> MGSSHHHHHHSQDPNSSMVKWYYKTITFLPELCNNESLAAKCLRVLHGFNYQYET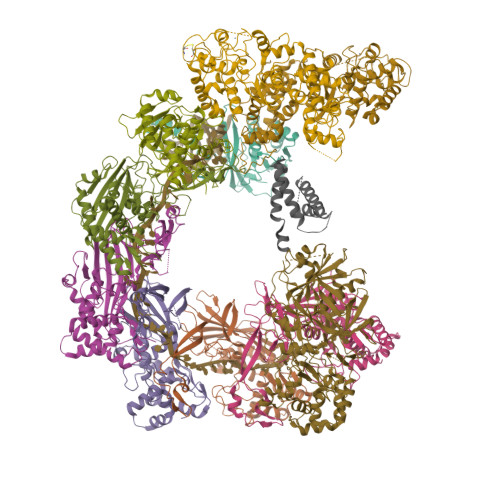RNIGVSFPLWCDATVGKKISFVSKNKIELDLLLKQHYFVQMEQLQYFHISNTVLVPEDCTYVSFRRCQSIDKLTAAGLARKIRRLEKRALSRGEQFDPSSFAQKEHTAIAHYHSLGESSKQTNRNFRLNIRMLSEQPREGNSIFSSYGLSNSENSFQPVPLI;> MQTLKELIASNPDDLTTELKRAFRPLTPHIAIDGNELDALTILVNLTDKTDDQKDLLDRAKCKQKLRDEKWWASCINCVNYRQSHNPKFPDIRSEGVIRTQALGELPSFLLSSSKIPPYHWSYSHDSKYVNKSAFLTNEFCWDGEISCLGELLKDADHPLWNTLKKLGCSQKTCKAMAKQLADITLTTINVTLAPNYLTQISLPDSDTSYISLSPVASLSMQSHFHQRLQDENRHSAITRFSRTTNMGVTAMTCGGAFRMLKSGAKFSSPPHHRLNSKRSWLTSEHVQSLKQYQRLNKSLIPENSRIALRRKYKIELQNMVRSWFAMQDHTLDSNILIQHLNHDLSYLGATKRFAYDPAMTKLFTELLKRELSNSINNGEQHTNGSFLVLPNIRVCGATALSSPVTVGIPSLTAFFGFVHAFERNINRTTSSFRVESFAICVHQLHVEKRGLTAEFVEKGDGTISAPATRDDWQCDVVFSLILNTNFAQHIDQDTLVTSLPKRLARGSAKIAIDDFKHINSFSTLETAIESLPIEAGRWLSLYAQSNNNLSDLLAAMTEDHQLMASCVGYHLLEEPKDKPNSLRGYKHAIAECIIGLINSITFSSETDPNTIFWSLKNYQNYLVVQPRSINDETTDKSSL;>[6x]MADLKLPTNLAYERSIDPSDVCFFVVWPDDRKTPLTYNSRTLLGQMEAASLAYDVSGQPIKSATAEALAQGNPHQVDFCHVPYGASHIECSFSVSFSSELRQPYKCNSSKVKQTLVQLVELYETKIGWTELATRYLMNICNGKWLWKNTRKAYCWNIVLTPWPWNGEKVGFEDIRTNYTSRQDFKNNKNWSAIVEMIKTAFSSTDGLAIFEVRATLHLPTNAMVRPSQVFTEKESGSKSKSKTQNSRVFQSTTIDGERSPILGAFKTGAAIATIDDWYPEATEPLRVGRFGVHREDVTCYRHPSTGKDFFSILQQAEHYIEVLSANKTPAQETINDMHFLMANLIKGGMFQHKGD;>[2x]MFLQRPKPYSDESLESFFIRVANKNGYGDVHRFLEATKRFLQDIDHNGYQTFPTDITRINPYSAKNSSSARTASFLKLAQLTFNEPPELLGLAINRTNMKYSPSTSAVVRGAEVFPRSLLRTHSIPCCPLCLRENGYASYLWHFQGYEYCHSHNVPLITTCSCGKEFDYRVSGLKGICCKCKEPITLTSRENGHEAACTVSNWLAGHESKPLPNLPKSYRWGLVHWWMGIKDSEFDHFSFVQFFSNWPRSFHSIIEDEVEFNLEHAVVSTSELRLKDLLGRLFFGSIRLPERNLQHNIILGELLCYLENRLWQDKGLIANLKMNALEATVMLNCSLDQIASMVEQRILKPNRKSKPNSPLDVTDYLFHFGDIFCLWLAEFQSDEFNRSFYVSRW>[4x]AEVPLPQLRAYTVDASWLQPMAPLQIADHTWQIGTEDL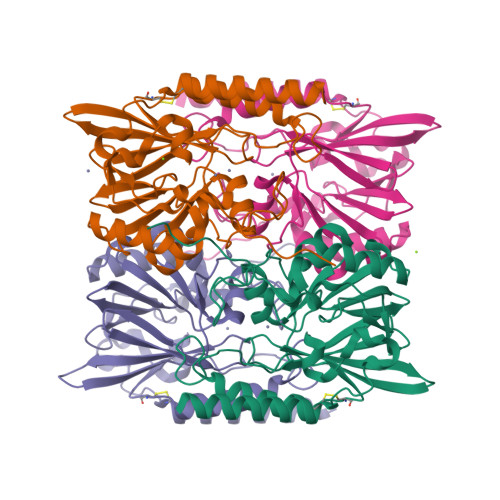TALLVQTPDGAVLLDGGMPQMASHLLDNMKARGVTPRDLRLILLSHAHACHAGPVAELKRRTGAKVAANAESAVLLARGGSDDLHFGDGITYPPANADRIVMDGEVITVGGIVFTAHFMAGHTPGSTAWTWTDTRNGKPVRIAYADSLSAPGYQLQGNPRYPHLIEDYRRSFATVRALPCDVLLTPHPGASNWDYAAGARAGAKALTCKAYADAAEQKFDGQLAKETAGAR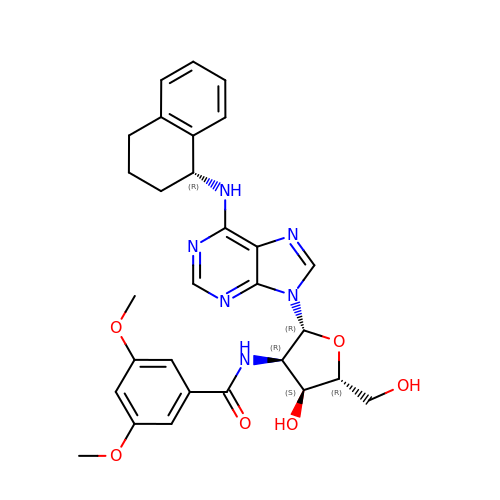N-1,2,3,4-TETRAHYDRONAPHTH-1-YL-2'-[3,5-DIMETHOXYBENZAMIDO]-2'-DEOXY-ADENOSINE | C29 H32 N6 O6 | FDZQGEIYGFPMOB-ZUURFMEUSA-N> QKPGETKEVHPQLTTFRCTKRGGCKPATNFIVLDSLSHPIHRAEGLGPGGCGDWGNPPPKDVCPDVESCAKNCIMEGIPDYSQYGVTTNGTSLRLQHILPDGRVPSPRVYLLDKTKRRYEMLHLTGFEFTFDVDATKLPCGMNSALYLSEMHPTGAKSKYNPGGAYYGTGYCDAQCFVTPFINGLGNIEGKGSCCNEMDIWEANSRASHVAPHTCNKKGLYLCEGEECAFEGVCDKNGCGWNNYRVNVTDYYGRGEEFKVNTLKPFTVVTQFLANRRGKLEKIHRFYVQDGKVIESFYTNKEGVPYTNMIDDEFCEATGSRKYMELGATQGMGEALTRGMVLAMSIWWDQGGNMEWLDHGEAGPCAKGEGAPSNIVQVEPFPEVTYTNLRWGEIGSTYQELQ

Though often considered synonymous with cellulases, β-1,4-glucanases are enzymes which recognize β-1,4-linked glucan chains which are characteristic of both the cellulosic and hemicellulosic (i.e. mixed-linkage glucans, xyloglucans, and glucomannans) fractions of plant biomass. The catalytic actions of a variety of retaining β-1,4-glucanases contribute to the breakdown of lignocellulosic polysaccharides. Humicola insolens Cel7B (HiCel7B) was chosen as a model β-d-glucanase since it is well-characterized, has good hydrolytic performance with chromogenic substrates, can be readily crystallised, and has been studied in our lab previously. As a tool for the rapid detection and identification of β-1,4-glucanases, a series of glycosylated cyclophellitol inhibitors mimicking β-1,4-glucan oligosaccharides have been synthesised.

The addition of another β-1,4-linked glucose residue to the non-reducing terminus to give 5 improved the performance of the inhibitor roughly 7-fold (ESI†), however intact MS with 2.2 μM enzyme and 5 μM inhibitor revealed minimal labelling (ESI†). Treatment with 5 gave small peaks with mass differences of both ∼338 Da (equivalent to addition of 1) and ∼500 Da (expected). Soaking HiCel7B crystals with 0.1 mM 5 also gave an unliganded enzyme structure. Repeating the intact MS experiment with a higher inhibitor concentration (50 μM) resulted in more overall labelling, but still a dominant mass difference of ∼338 Da. Lowering the inhibitor (5 μM) and enzyme concentrations (0.5 μM) gave overall weaker signal, showing incomplete labelling, with a mass difference attributable to 5 as the dominant modification (ESI†). We interpret these results as indicative of an internal hydrolysis of 5 to give primarily a mixture of cellobiose and cyclophellitol, which is unreactive, and secondarily a mixture of 1 and glucose, which gives rise to the smaller observed mass difference. The observed concentration-dependence suggests that both hydrolytic processes have a higher KM than the KI of the interaction between HiCel7B and 5. Thus, the course of inhibition of HiCel7B with 5 is enzyme- and inhibitor concentration-dependent, being affected by the KM of the two possible hydrolytic pathways and the KI values for 5 and 1.>MAMNKQNNYSDDSIQVLEGLEAVRKRPGMYIGSTDKRGLHHLVYEIVDNSVDEVLNGYGNEIDVTINKDGSISIEDNGRGMPTGIHKSGKPT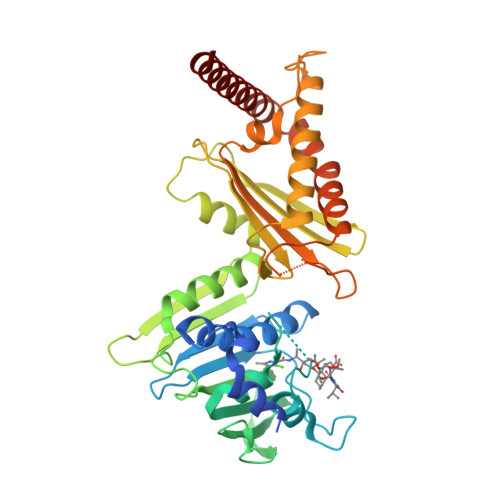VEVIFTVLHAGGKFGQGGYKTSGGLHGVGASVVNALSEWLEVEIHRDGNIYHQSFKNGGSPSSGLVKKGKTKKTGTKVTFKPDDTIFKASTSFNFDVLSERLQESAFLLKNLKITLNDLRSGKERQEHYHYEEGIKEFVSYVNEGKEVLHDVATFSGEANGIEVDVAFQYNDQYSESILSFVNNVRTKDGGTHEVGFKTAMTRVFNDYARRINELKTKDKNLDGNDIREGLTAVVSVRIPEELLQFEGQTKSKLGTSEARSAVDSVVADKLPFYLEEKGQLSKSLVKKAIKAQQAREAARKAREDARSGKKNKR[2x]>[55x]MGLFDRIKRVVSSNLNDLVNKAEDPEKMLEQAILEMQEDLVQLRQGVAQAIAAQKRSEKQYNDAQNEINKWQRNAQLALQKGDENLARQALERKKTYTDTSAALKASLDTQSTQVETLKRNLIQLESKISEAKTKKEMLKARITTAKAQEQLQGMVRGMNTSSAMSAFERMEEK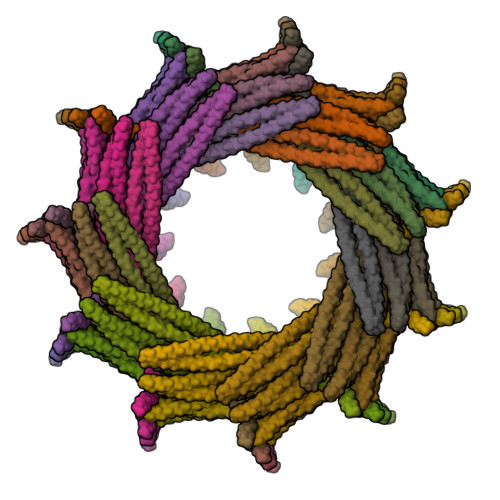VLMQESRAQALGELAGADLETQFAQLEGGSDVDDELAALKAQMLPPATPVTQAQLPPQQETTPAKSNEVVDAELDSLRKQLDQL N-(2-ethoxy-3,5-dimethylbenzyl)-1H-tetrazol-5-amine | C12 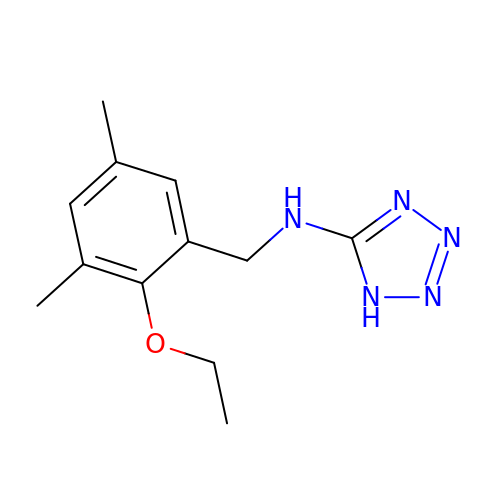H17 N5 O | WHEQZFWVEMEFGH-UHFFFAOYSA-N>[2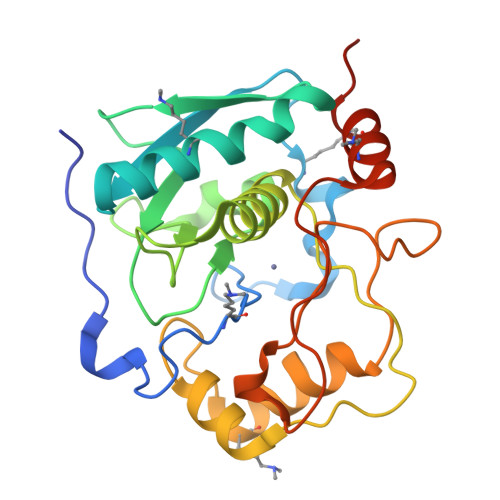x]MDSSKGLKELRAVPKADIVSGFEGAKVCKDVYPKGTDPRGAVVRSTKWPNGSVITVGLYGGTPYVRSKVKQYAQEWSNYANITFNFVESGTPQIRVTFTQGAGSYSYLGTQALSIPSNEETMNFGWFDDSTSDTEFSRTVIHEFGHALGMIHEHQHPLTNIPWDKNKVYAYYAGYPNYWSKKDVDNNLFATYSTTQTQYSAYDTQSIMHYSISSALTTNGFSVGNNSVLSATDKQFIATVYPRNLEHHHHHH> AECSVDIQGNDQMQFNTNAITVDKSCKQ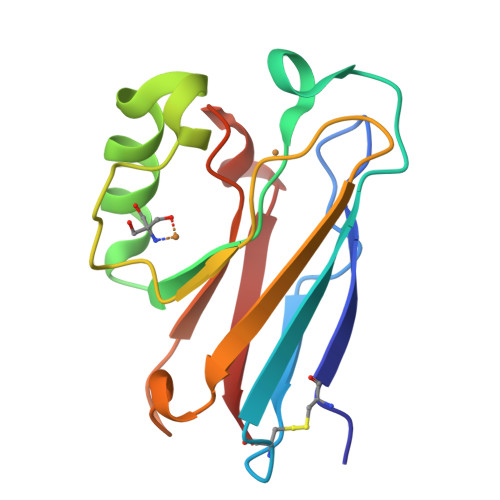FTVNLSHPGNLPKNVMGHNWVLSTAADMQGVVTDGMASGLDKDYLKPDDSRVIAHTKLIGSGEKDSVTFDVSKLKEGEQYMFFCTFPFHSALMKGTLTLK> GPLGSTAFRKFYERGDFPIALEHDSKGNKIAWKVEIEKLDYHHYLPLFFDGLCEMTFPYEFFARQGIHDMLEHGGNKILPVLPQLIIPIKNALNLRNRQVICVTLKVLQHLVVSAEMVGKALVPFYRQILPVLNIFKNMNVNSGDGIDYSQQKRENIGDLIQETLEAFERYGGENAFINIKYVVPTYESCLLN;> GPLGSMASSDVKPKSVSHAKKW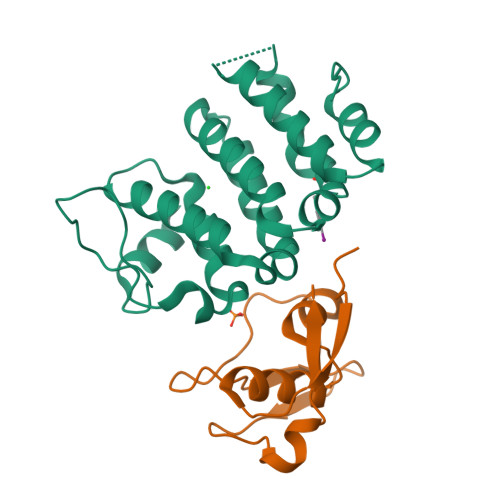SEEIENLYRFQQAGYRDETEYRQVKQVSMVDRWPETGYVKKLQRRDNTFYYYNKQRECDDKEVHKVKIYAY1-(5-bromanylpyridin-3-yl)-4-[4-(3-methylphenyl)cyclohexyl]piperazin-4-ium | C22 H29 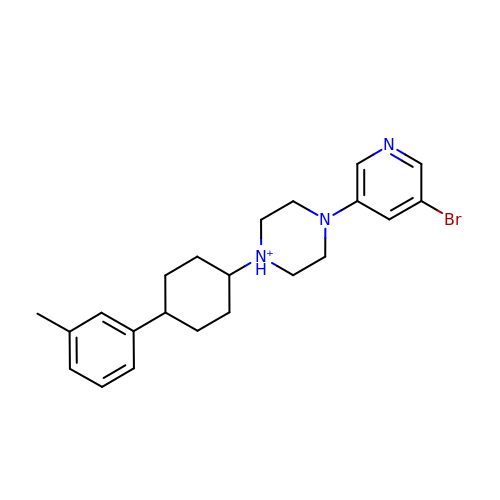Br N3 | GPGOZHVXQXMXPF-XGAFWQRZSA-O[[(2~{R},3~{S},4~{R},5~{R})-3,4-bis(oxidanyl)-5-(6-oxidanylidene-1~{H}-purin-9-yl)oxolan-2-yl]methoxy-oxidanyl-phosphoryl] 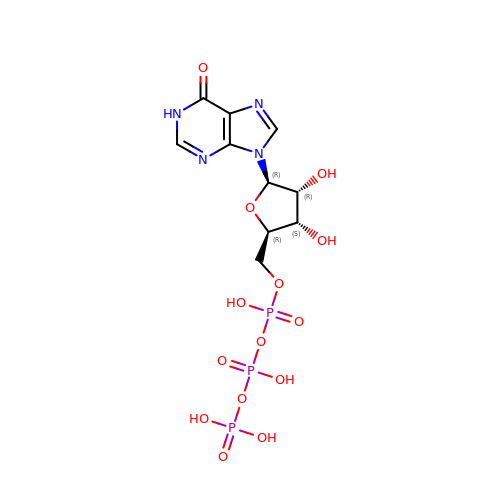phosphono hydrogen phosphate | C10 H15 N4 O14 P3 | HAEJPQIATWHALX-KQYNXXCUSA-N> GAMAGKKVLIVYAHQEPKSFNGSLKNVAVDELSRQGCTVTVSDLYAMNFEPRATDKDITGTLSNPEVFNYGVETHEAYKQRSLASDITDEQKKVREADLVIFQFPLYWFSVPAILKGWMDRVLCQGFAFDIPGFYDSGLLQGKLALLSVTTGGTAEMYTKTGVNGDSRYFLWPLQHGTLH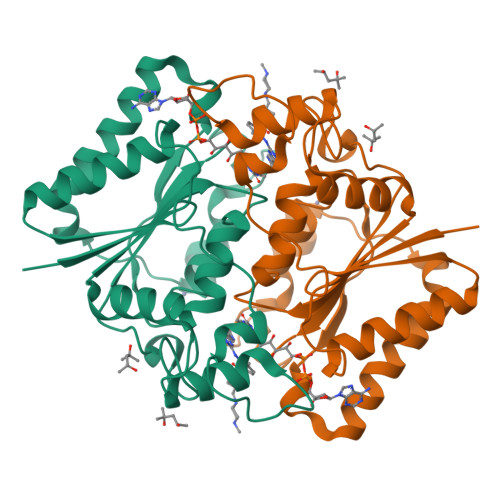FCGFKVLAPQISFAPEIASEEERKGMVAAWSQRLQTIWKEEPIPCTAHWHFGQ>[4x]MPEIITPIITPFTKDNRIDKEKLKIHAENLIRKGIDKLFVNGTTGLGPSLSPEEKLENLKAVYDVT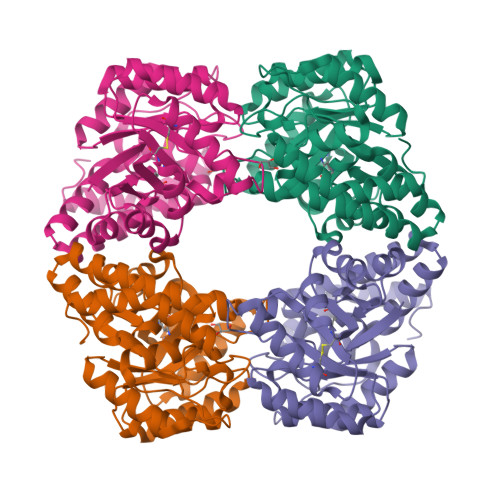NKIIFQVGGLNLDDAIRLAKLSKDFDIVGIASYAPYYYPRMSEKHLVKYFKTLCEVSPHPVYLYNYPTATGKDIDAKVAKEIGCFTGVKDTIENIIHTLDYKRLNPNMLVYSGSDMLIATVASTGLDGNVAAGSNYLPEVTVTIKKLAMERKIDEALKLQFLHDEVIEASRIFGSLSSNYVLTKYFQGYDLGYPRPPIFPLDDEEERQLIKKVEGIRAKLVELKILKE> MLKQVEIFTDGS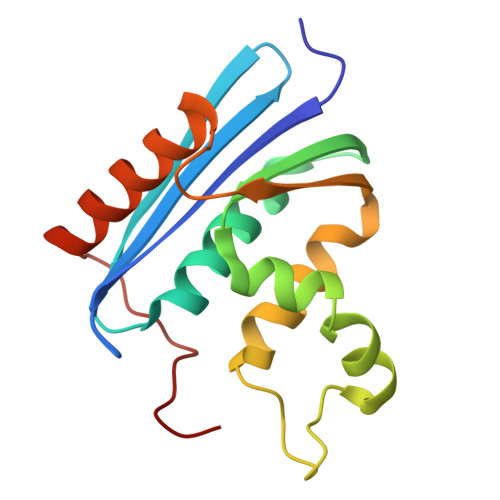CLGNPGPGGYGAILRYRGREKTFSAGYTRTTNNRMELMAAIVALEALKEPCEVILSTDSQYVRQGITQWIHNWKKRGWKTADKKPVKNVDLWQRLDAALGQHQIKWEWVKGHAGHPENERCDELARAAAMNPTLEDTGYQVEV In Saccharomyces cerevisiae, the pre-mRNA leakage 39-kDa protein (ScPml39) was reported to retain unspliced pre-mRNA prior to export through nuclear pore complexes (NPCs). ScPml39 is required for cell growth in the absence of a functional Y-complex, an essential NPC building block required for mRNA export, and is recruited to the nuclear basket of NPCs by virtue of interactions with the N-terminal regions of ScMlp1 and ScMlp227. The crystal structure revealed integrated zf-C3HC and Rsm1 modules, which are tightly associated through a hydrophobic interface to form a single domain. Both zf-C3HC and Rsm1 modules belong to the Zn-containing BIR (Baculovirus IAP repeat)-like super family, with key residues of the canonical BIR domain being conserved.

Based on the domain boundaries identified by mass spectrometry, we generated a truncated ScPml39 construct comprising residues 77–317 for structural studies. ScPml3977–317 was crystalized in the P3121 space group. The phases and the structure were determined to a resolution of 2.5 Å by Zinc single-wavelength anomalous dispersion (Zn-SAD). The majority of the fragment (residues 79–311) was well resolved in the electron density, while no electron density was observed for two N-terminal residues (77–78), residues 148–151 between β3 strand and helix αC, a Ser-rich region comprising residues 213–226, and six C-terminal residues (312–317). ScPml3977–317 contains two BIR-like modules: zf-C3HC (residues 79–189 in blue) and Rsm1 (residues 190–311 in purple). The two zf-C3HC and Rsm1 modules form a single structural domain stabilized by the hydrophobic residues Leu87, Ile90, Pro111, Leu112, Leu185, Tyr189 of zf-C3HC and Tyr190, Phe272, and Trp291 of Rsm1. Cys134, Cys137, His172, and Cys176 residues coordinate Zn to form the C-x2-C-x–H-x3-C ZnF motif. Due to the different spacing within the CCHC ZnF motif, helix αC of the ScPml39 zf-C3HC module is tilted by 42° with respect to the corresponding helix αC in D. melanogaster IAP1-BIR1 domain, rendering the distinct spacing a key determinant for the topology of ScPml39. Cys268, Cys271, His288, and Cys292 coordinate Zn and are part of the C-x2-C-x16-H-x3-C ZnF motif. Thus, the distinct CCHC ZnF spacing between Zn-coordinating residues and helix αAB′ insertion between helices αA′ and αΒ′ represent key determinants of the Rsm1 module.

> GPHMAMGFRLHDLRALLKRICSIQNYTRHVLIEWDVRWVNPLTLASKGWEPYQSASQSQVPFKCCCCHAIMTIPLLKNGDDVADYTMKLNEKIWNSNIIGNHLQKCPWRENQVDLNKEYYLSSQNLIREIERIHTEIDRIVSGSNEFSLKRNSSRIFHYLSEKEIQKLAFFFDCKDYSLVGLLLLGYTKFQKDDLVQCTACFHRASLKKLEYTEFNGHALWCRYYNKELLPTMLLELIGKEDKLITK> TNGTMMQYFEWHLPNDGQHWNRLRDDASNLRNRGITAIWIPPAWKGTSQNDVGYGAYDLYDLGEFNQKGTVRTKYGTRSQLESAIHALKNNGVQVYGDVVMNHKGGADATENVLAVEVNPNNRNQEISGDYTIEAWTKFDFPGRGNTYSDFKWRWYHFDGVDWDQSRQFQNRIYKFRGDGKAWDWEVDSENGNYDYLMYADVDMDHPEVVNELRRWGEWYTNTLNLDGFRIDAVKHIKYSFTRDWLTHVRNATGKEMFAVAEFWKNDLGALENYLNKTNWNHSVFDVPLHYNLYNASNSGGNY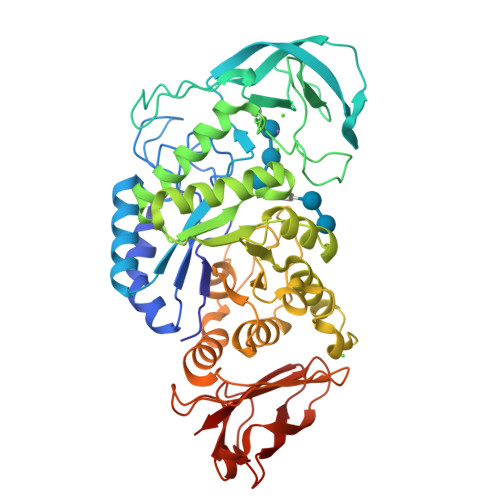DMAKLLNGTVVQKHPMHAVTFVDNHDSQPGESLESFVQEWFKPLAYALILTREQGYPSVFYGDYYGIPTHSVPAMKAKIDPILEARQNFAYGTQHDYFDHHNIIGWTREGNTTHPNSGLATIMSDGPGGEKWMYVGQNKAGQVWHDITGNKPGTVTINADGWANFSVNGGSVSIWVKR>MDKGKSVKSTEKSVGMPPKTPKTDNNAHVDNEFLILQVNDAVFPIGSYTHSFGLETYIQQKKVTNKESALEYLKANLSSQFLYTEMLSLKLTYESALQQDLKKILGVEEVIMLSTSPMELRLANQKLGNRFIKTLQAMNELDMGEFFNAYAQKTKDPTHATSYGVFAASLGIELKKALRHYLYAQTSNMVINCVKSVPLSQNDGQKILLSLQSPFNQLIEKTLELDESHLCTASVQNDIKAMQHESLYSRLYMS[2x];>[2x]MNTYAQESKLRL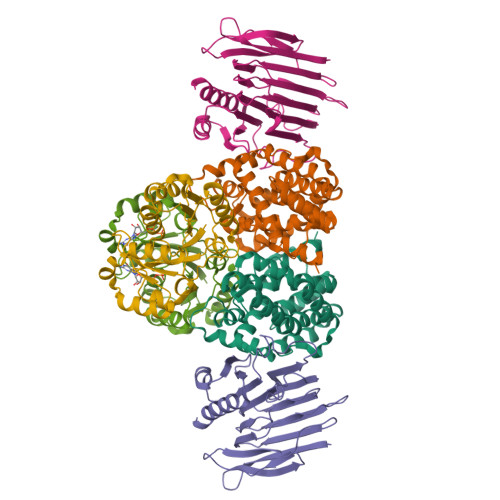KTKIGADGRCVIEDNFFTPPFKLMAPFYPKDDLAEIMLLAVSPGMMRGDAQDVQLNIGPNCKLRITSQSFEKIHNTEDGFASRDMHIVVGENAFLDFAPFPLIPFENAHFKGNTTISLRSSSQLLYSEIIVAGRVARNELFKFNRLHTKISILQDEKPIYYDNTILDPKTTDLNNMCMFDGYTHYLNLVLVNCPIELSGVRECIEESEGVDGAVSETASSHLCVKALAKGSEPLLHLREKIARLVTQTTTQKV;>[2x]MVKIGVCGPVGSGKTALIEALTRHMSKDYDMAVITNDIYTKEDAEFMCKNSVMPRERIIGVETGGCPHTAIREDASMNLEAVEEMHGRFPNLELLLIESGGDNLSATFNPELADFTIFVIDVAEGDKIPRKGGPGITRSDLLVINKIDLAPYVGADLKVMERDSKKMRGEKPFIFTNIRAKEGLDDVIAWIKRNALLED>[3x]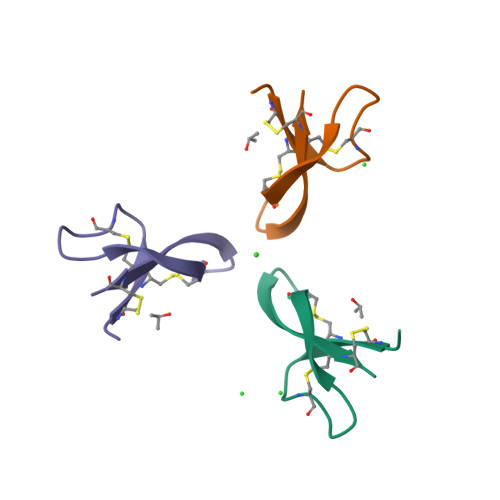ATCYCRTGRCATRESLSGVCEISGRLARLCCR> MTWEKGEEIVKQILEKAPYAEGKVRRERRLEFRVPADKIRDFLRIMKESNFPLMLQITAVDWPKEGEIELVYHLINVELGTHAMVKTRIPRDLDKARMPTVKDIYPAAETYERDVHDFFGVYFEGNEKMEMPWILDDPERGLYPHRKDFDMLA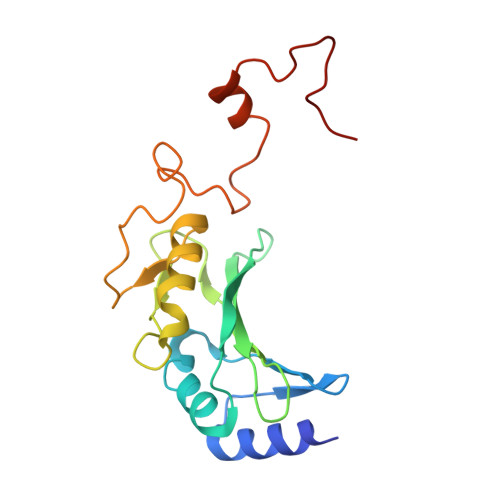YVKKKYKILDRFDEDKDKYVI N~6~-(2,6-dichlorophenyl)-N~6~-(pent-2-yn-1-yl)quinoline-4,6-diamine 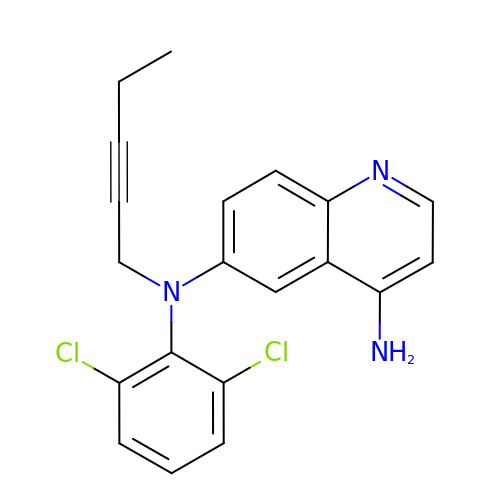| C20 H17 Cl2 N3 | XBWBLXQDIZDDLL-UHFFFAOYSA-N N-(1-{[(3-methylbenzoyl)amino]methyl}cyclopentyl)-2,1-benzoxazole-4-carboxamide | C22 H23 N3 O3 | 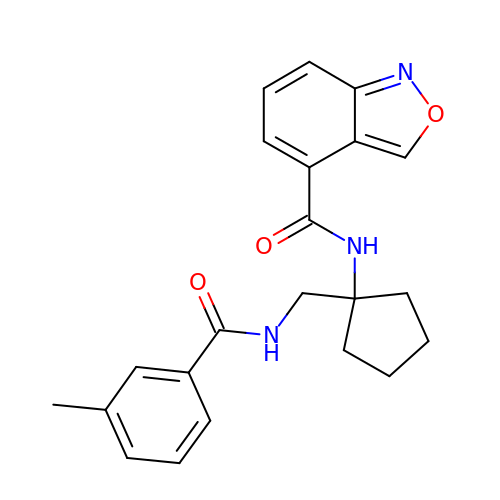MHXAYWIKTBXLMI-UHFFFAOYSA-N>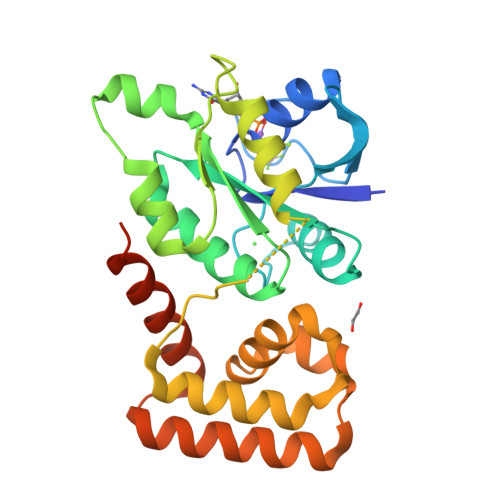[2x]GAMASHMTEIALIGNPNSGKTSLFNLITGHNQRVGNWPGVTVERKSGLVKKNKDLEIQDLPGIYSMSPYSPAAKVARDYLLSQRADSILNVVDATNLERNLYLTTQLIETGIPVTIALNMIDVLDGQGKKINVDKLSYHLGVPVVATSALKQTGVDQVVKKAAHTTTSTVGDLAFPIYDDRLEAAISQILEVLGNSVPQRSARFYAIKLFEQDSLVEAELDLSQFQRKEIEDIIRITEEIFTEDAESIVINERYAFIERVCQMAESHTEDFALTLS> MAHHHHHHMSEPRKILVTSALPYANGSIHLGHMLEYIQTDMWVRFQKMRGNQAVYVCADDAHGSAIMLRAEREGITSEQLIDAVRAEHMGDFADFLVDFDNYHSTHSEENRELSSAIYLKLRDAGHIDTRPVTQYFDPEKQMFLADRFIKGTCPKCGTADQYGDNCEACGATYAPTELKDPKSAISGATPVLKESLHYFFKLPDFEAMLKQWTRSGALQESVANKLAEWLDSGLQQWDISRDAPYFGFEIPDAPGKYFYVWLDAPIGYMASFKNLCARRPELDFDAFWGKDSGAELYHFIGKDIVNFHALFWPAMLEGAGYRKPTALNVHGYLTVNGQKMSKSRGTFVKARTYLDHLDPEYLRYYYASKLGRGVEDLDLNLEDFVQKVNSDLVGKVVNIASRCAGFIHKGNAGVLVGADPAPELLAAFREAAPGIAEAYEARDFNRAMREIMALADRANAWIAEQAPWALAKQEGQQDKVQAVCGLGINLFRQLVIFLKPVLPK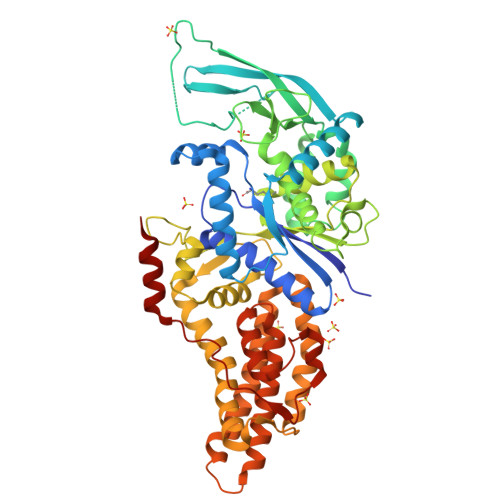LAAAAEAFLNVAPLTWADHQTLLANHQLNPFQPLMTRIEPAKVEAMIEASKEDLA>SLEVIIKAKVKPTEDKYKVKKAIL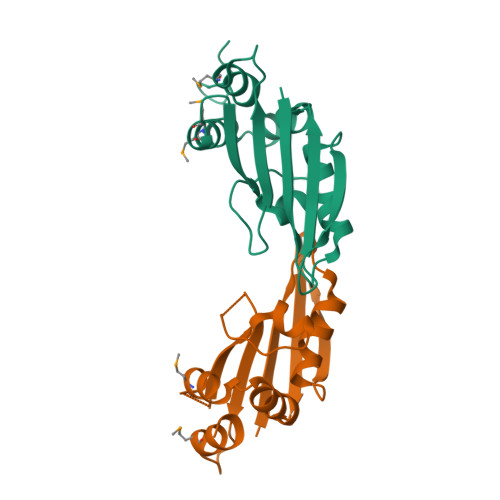NIFPKAKLTFIEKDNEFGEWEGKTKSVEKLKELLRSQSILDAARMVLEKGMTENATKFYLNKQAAYVGAVNFDIDTHGGIFVKILADENEDIMKIIKDIAPRTKGGVIINEDELEEGHHHHHH[4x]>PELPEVETTRRRLRPLVLGQTLRQVVHRDPARYRNTALAEGRRILEVDRRGKFLLFALEGGVELVAHLGMTGGFRLEPTPHTRAALVLEGRTLYFHDPRRFGRLFGVRRGDYREIPLLLRLGPEPLSEAFAFPG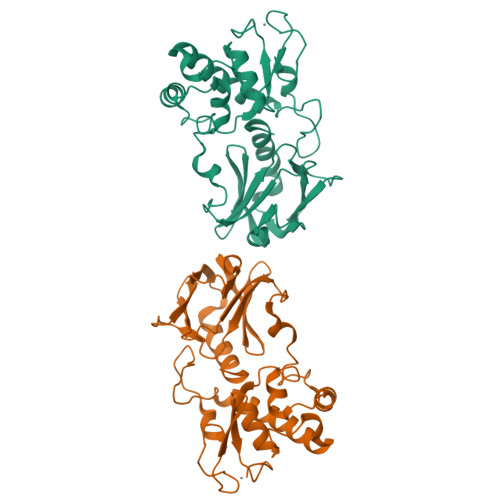FFRGLKESARPLKALLLDQRLAAGVGNIYADEALFRARLSPFRPARSLTEEEARRLYRALREVLAEAVELGGSTLSDQSYRQPDGLPGGFQTRHAVYGREGLPCPACGRPVERRVVAGRGTHFCPTCQGEGP[2x]> RSVYELDCIPLWGTVSIQGNASEMEAAFAVSPHFLKLPIKMLMGDHEGMSPSLTHLTGHFFGVYDGHGGHKVADYCRDRL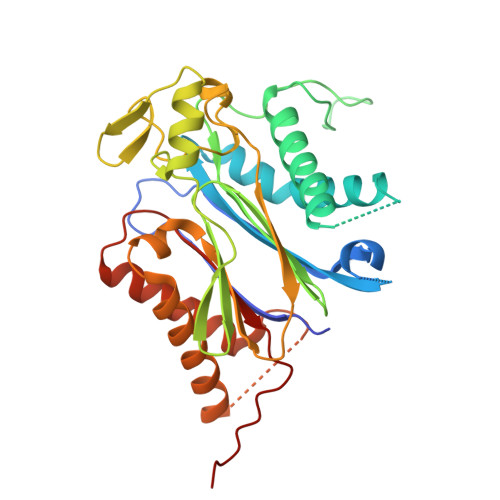HFALAEEIERIKDELCKRNTGEGRQVQWDKVFTSCFLTVDGEIEGKIGRAVVGSSDKVLEAVADETVGSTAVVALVCSSHIVVSNCGDSRAVLFRGKEAMPLSVDHKPDREDEYARIENAGGKVIQWQGARVFGRLAMSRSIGDRYLKPYVIPEPEVTFMPRSREDECLILASDGLWDVMNNQEVCEIARRRILMWHKKNGAPPLAERGKGIDPACQAAADYLSMLALQKGSKDNISIIVIDLKAQRKFKTAT>[2x]MVLYFIGLGLYDERDITVMGLEIAKKCDYVFAEFYT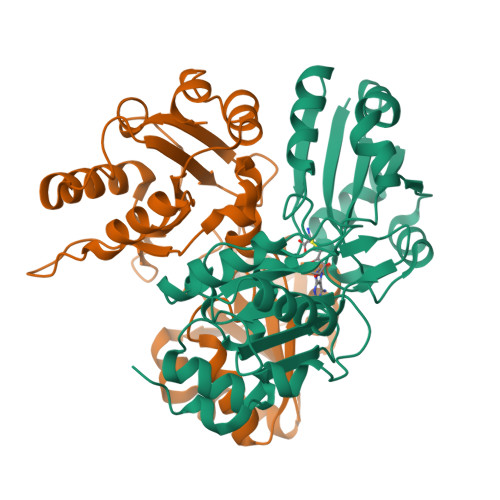SLMAGTTLGRIQKLIGKEIRVLSREDVELNFENIVLPLAKENDVAFLTPGDPLVATTHAELRIRAKRAGVESYVIHAPSIYSAVGITGLHIYKFGKSATVAYPEGNWFPTSYYDVIKENAERGLHTLLFLDIKAEKRMYMTANEAMELLLKVEDMKKGGVFTDDTLVVVLARAGSLNPTIRAGYVKDLIREDFGDPPHILIVPGKLHIVEAEYLVEIAGAPREILRVNV> LGKKPIYKKA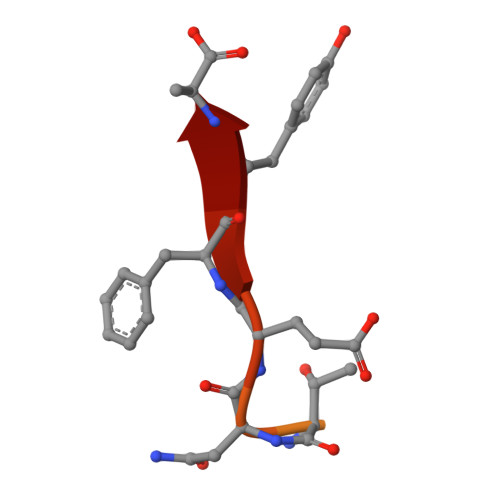PTNEFYA> AVEPKEDTITVTAAPAPQESAWGPAATIAARQSATGTKTDTPIQKVPQSISVVTAEEMALHQPKSVKEALSYTPGVSVGTRGASNTYDHLIIRGFAAEGQSQNNYLNGLKLQGNFYNDAVIDPYMLERAEIMRGPVSVLYGKSSPGGLLNMVSKRPTTEPLKEVQFKAGTDSLFQTGFDFSDSLDDDGVYSYRLTGLARSANAQQKGSEEQRYAIAPAFTWRPDDKTNFTFLSYFQNEPETGYYGWLPKEGTVEPLPNGKRLPTDFNEGAKNNTYSRNEKMVGYSFDHEFNDTFTVRQNLRFAENKTSQNSVYGYGVCSDPANAYSKQCAALAPADKGHYLARKYVVDDEKLQNFSVDTQLQSKFATGDIDHTLLTGVDFMRMRNDINAWFGYDDSVPLLNLYNPVNTDFDFNAKDPANSGPYRILNKQKQTGVYVQDQAQWDKVLVTLGGRYDWADQESLNRVAGTTDKRDDKQFTWRGGVNYLFDNGVTPYFSYSESFEPSSQVGKDGNIFAPSKGKQYEVGVKYVPEDRPIVVTGAVYNLTKTNNLMADPEGSFFSVEGGEIRARGVEIEAKRPLSASVNVVGSYTYTDAEYTTDTTYKGNTPAQVPKHMASLWADYTFFDGPLSGLTLGTGGRYTGSSYGDPANSFKVGSYTVVDALVRYDLARVGMAGSNVALHVNNLFDREYVA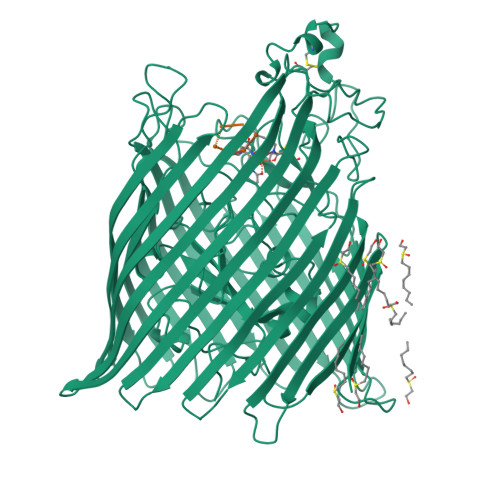SCFNTYGCFWGAERQVVATATFRF;> AAAGGG> MSGLSDFFTQLGQDAQLMEDYKQNPEAVMRAHGLTDE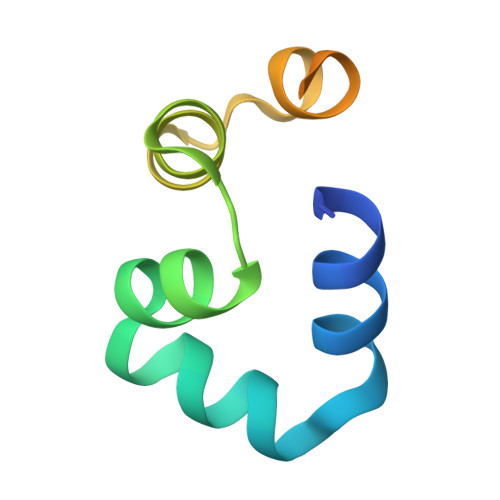QINAVMTGDMEKLKTLSGDSSYQSYLVISHGNGD>MGHHHHHHSHMRTLAVISAGLSTPSSTRQIADSISEAVTAAVSARGEALSVSTIELSELIPDLMTAMTTRVHTTKLEEI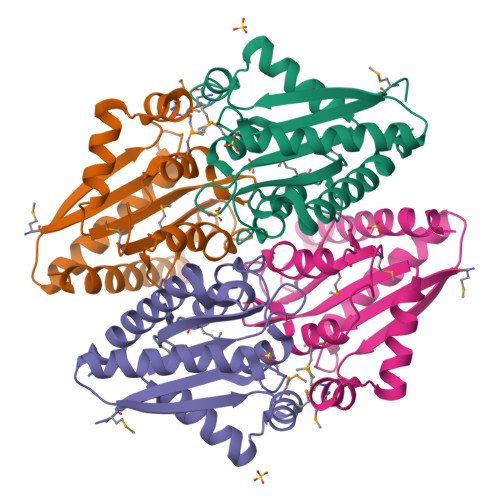TSALSASDGLVVATPVFKASYTGLFKMFFDILDTDALTGMPTIIAATAGSARHSLVLDYALRPLLSYMRAVVVPTGVFAATEDFGGPEGAEFNKRIARAAGELASLIVEESG[6x]Neisserial adhesin A (NadA) is one of the main vaccine antigens, acts in host cell adhesion, and may influence colonization and invasion. NadA belongs to the OCA (oligomeric coiled-coil adhesin) family, a subgroup of the trimeric autotransporter adhesins (TAA), which generally mediate adhesion of Gram-negative bacteria to target cells or to the extracellular matrix and invasion. Similarly, recombinant NadA was reported to stimulate human monocytes by binding Hsp90 (26, 27). It was recently demonstrated that the NadA3 N-terminal region binds specifically to the endothelial cell receptor LOX-1 (low-density oxidized lipoprotein lectin-like receptor 1). The structure of NadA3 24–170 presents a small globular head region (residues 24 to 85) and a long trimeric coiled-coil motif made of canonical heptad repeats, plus the two novel undecad repeats.

Through a cavity-filling mutagenesis approach on NadA3, we identified the mutations A33I, I38L, and A39V, all of which increased thermostability, with the A33I I38L double mutation conferring a remarkable 17°C Tm increase. Next, we performed structural studies to verify the organization of the most highly stabilized mutant; we crystallized and determined the structure of the NadA3 24–170 A33I I38L double mutant. The structure was refined to a resolution of 2.65 Å, with final Rwork and Rfree values of 20% and 24%. Upon superposition, the mutant structure was confirmed to be essentially identical to that of the native protein, even in the relatively flexible wings, exhibiting a root mean square deviation (RMSD) of 0.23 Å for the pairwise superposition of 144 Cα atoms. Moreover, the residues mutated to I33 and L38 present unchanged backbone positions and more-extensive van der Waals’ interactions mediated by their side chains than the original Ala and Ile residues in the native structure. Therefore, the crystal structure of the double mutant confirmed that improved filling of the cavity with hydrophobic residues had successfully created a stabilized antigen. The halide ion, coordinated by Asn44 side chains and >9 Å away from both mutated residues, was present in the same position and with full occupancy in both structures. The halide in the stabilized mutant presented a lower B factor than in the wild type (44.6 Å2 versus 69.7 Å2), which likely reflects a higher overall stability in the mutant, which has a lower overall B factor than the wild type (66.0 Å2 versus 88.3 Å2). However, some mutations abolished binding to LOX-1; these were A33I, A33I I38L, and Y42A. While the presence of the bulky Ile side chain at position 33 in NadA4 and NadA5 may confer greater thermostability, it may also cause the functional closure of this intermonomer pocket, resulting in the observed loss of binding to LOX-1.

>[3x]ATNDDDVKKIATVALAAAYNNGQEINGFKAGETIYDIDEDGTITKKDATAADVEADDFKGLGLKKVVTNLTKTVNENKQNVDAKVKAAESEIEKLTTKLADTDAALADTDAALDATTNALNKLGENITTFAEETKTNIVKIDEKLEAASKHHHHHH> MAHHHHHHMNAFIEELKWRGLWADMTPGTEDQLNKEMTTAYIGFDPTADSLHIGSLIPIKILAHFQRHGHKPIALVGGATGMIGDPSGKSAERNLLDEETLLYYVDCLKNQLSRFLDFEGDGPNRAELVNNYDWMKNVTFLDFAKNIGKHITVNYMMAKDSVKKRFSGEDGADGMSFTEFTYQLLQGYDYLHLYKEKGVKLQMGGSDQWGNITTGTELIRRKAQGEAF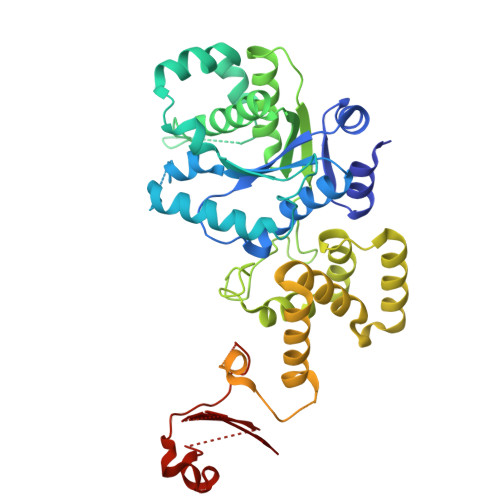ALTTKLITKADGSKFGKSESGENYWLDAKRTSPYRFYQFWLNATDEDGERFIKFYTFLEKEEIDKLIEEHRTAPHERKLQKKLAEEVTVWVHGRAEYKRALKASEILFGRSTAEDLVSLDEELFLQIFDGVPQKEVAKSEVIGSNIVDLISDKSGFLKSKGEAKRELTGNAISVNKEKVNDTFEVSEKDLIDGKFLLLQKGKKSYFIVKTVXXXXXXXXXXXXXXXXXXXXXXXXXXXXXXXXXXXXXXXXX{3-[(3aR,4R,5S,6aR)-4-azaniumyl-4-carboxyoctahydrocyclopenta[b]pyrrol-1-ium-5-yl]propyl}(trihydroxy)borate(1-) | C11 H24 B N2 O5 | 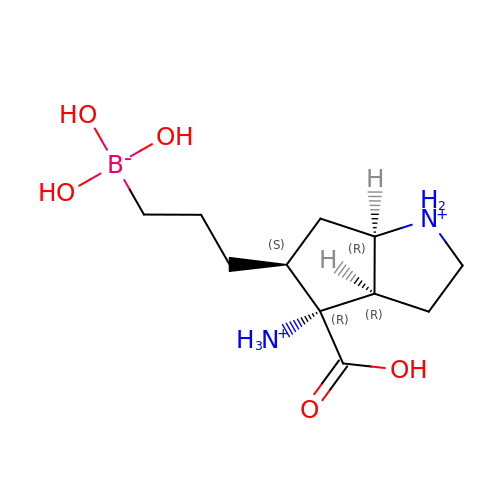ZNCURAYGFUECIT-YSSBGUOXSA-P In the Siphoviridae SPP1 phage, the tail tube consists of the TTPs gp17.1 and gp17.1* in a ratio of 3:1, with the latter being generated by a translational frameshift adding a fibronectin type III (FN3) domain to the C-terminus of the protein. However, virions only containing gp17.1 are still viable and infectious, indicating that the additional C-terminal FN3 domain is dispensable for phage assembly and infection. gp17.1 monomers are unstable in solution and spontaneously self-polymerize into long tubes in vitro which are indistinguishable from native tubes. Six gp17.1 subunits assemble into a ring with the inner 24 β-strands forming a β-barrel that defines the inner lumen of the tube. The α-helices are arranged almost parallel to the tail tube axis. These rings stack onto each other with a rotation of 21.9° forming a right-handed helical, hollow tube.

For cryo-EM experiments, we purified ΔN−3 gp17.1 which is indistinguishable from wt gp17.1 as judged by solid-state NMR. Curvy tubes were observed in the micrographs. For image processing those tubes that appeared most straight were selected. 3D reconstruction (see “Methods” section) yielded a density map with an average resolution of 4.3 Å. The local resolution varies significantly, from about 3.5 Å at the inner ring where the β-strands are well resolved, to worse than 5 Å at the periphery. The inner β-barrel shows nearly no motion on these timescales—which correlates with these areas being highest resolved in the cryo-EM density. The global, collective nature of this motion does not impose heterogeneity onto the cryo-EM map since only straight tubes are considered for structure calculation. In the context of the tail tube complex the C-arm of the superjacent subunit folds onto the outer β-sheet of the β-sandwich fold by anchoring the sidechain of Gln162 into a pocket. This interaction obscures the lipophilic area whereupon the complex is stabilized, because the number of unfavorable hydrophobic contacts with the solvent is reduced. Overall, our hybrid data support a model where the C-arm (143–176) and the loop (40–59) act as bellows contributing to tail tube bending by stretching.

>[12x]MPIMGQDVKYLFQSIDAATGSAPLFPAYQTDGSVSGERELFDEQTKNGRILGPGSVADSGEVTYYGKRGDAGQKAIEDAYQNGKQIKFWRVDTVKNENDKYDAQFGFAYIESREYSDGVEGAVEISISLQVIGELKNGEIDTLPEEIVNVSKGGYDFQQPGQTTGEAPGTVPAPHHHHHH>CDQKVADTTQASQKLAEPITVKHALGTTVIDHLPQRVAVLDMNEADFLDQLNVPIMGMPKDYVPHFLEKYKKDAQIQDLGAIVQPNMERIYALKPDLILMTPLHVNQYQELSKIAPTIHYDINFNNSESNHIGLVKDHMMTLGKIFNKEDLARQKVSELDEQVKQVQAVTANRPERALVVLHNNGAFSNFGIQSRYGFIFNAFGVKPASGVVDTSLHGQPISSEFIKKADPDILYIVDRTAVMEHRPNINAASVENPLLRQTKA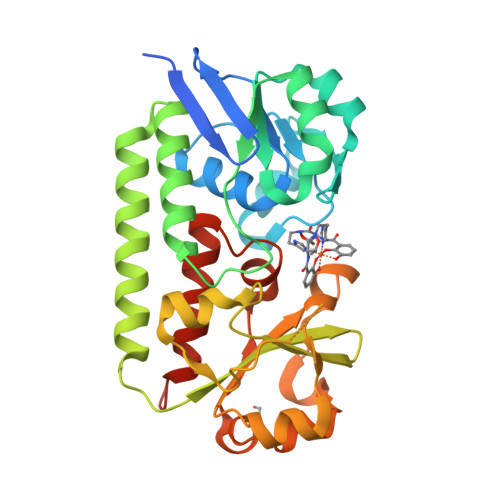WKNGRVIFVDADAWYTTAASPTSLKIVMEDVKKGYQLEHHHHHH[2x]>[2x]TRFTEEYQLFEELGKGAFSVVRRCVKVLAGQEYAAKIINTKKLSARDHQKLEREARICRLLKHPNIVRLHDSISEEGHHYLIFDLVTGGELFEDIVAREYYSEADASHCIQQILEAVLHCHQMGVVHRNLKPENLLLASKLKGAAVKLADFGLAIEVEGEQQAWFGFAGTPGYLSPEVLRKDPYGKPVDLWACGVILYILLVGYPPFWDEDQHRLYKQIKAGAYDFPSPEWDTVTPEAKDLI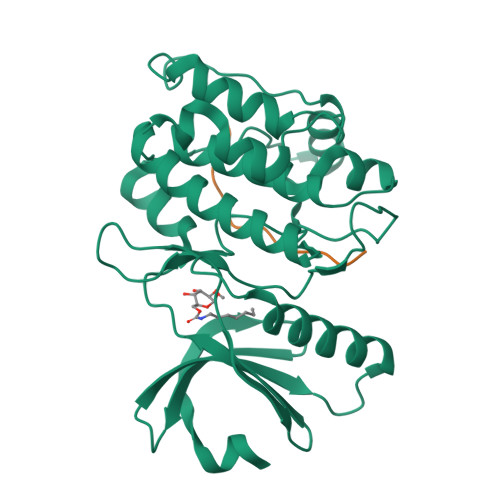NKMLTINPSKRITAAEALKHPWISHR;>[2x]KAQKKNRNKLRRQHDYDTFVDL> KDAQAIAKDMYPGWNLGNTLEATGSGLDAETSWQPTLTTQQIIDAVKAAGFKSVRIPCSWDIHSDSNGEIDAQWMARVKQVVNYCI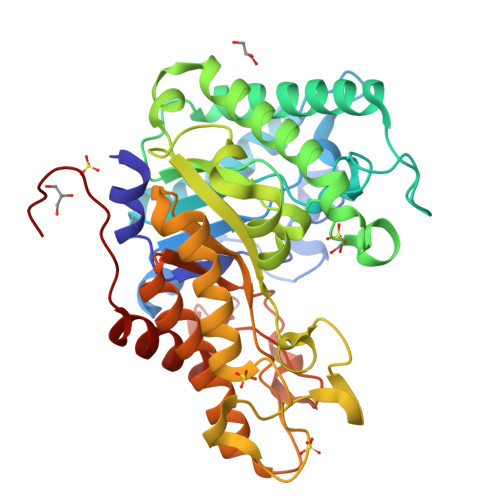NDGIYVVLNDHWDNGWIEVLGFSKSSSSYQAVDEATITSKITRLKDLWTQIANEFKDYDEHLLFAGLNEPFQEYSLFSGHHEELTPILCRYNQAFVEAVRATGGNNAQRTLVVQGPSTNINSSVNYMTADKLPETAGRLMVEVHYYDPGQFCGTFDASGDNAFYFWGAANHSTDHNATYGEEAYMLSQFGLLKTAYTSLGYPVIIGEYAALQRTISGDQNKHNASVKYFYQCVNEYATNNGIIAFAWDTNDTNGLNSEGGSSTIIDRANSAVVGNNAMEGVKAGVAAGKWPFLEHHHHHH> SMQEEDTFRELRIF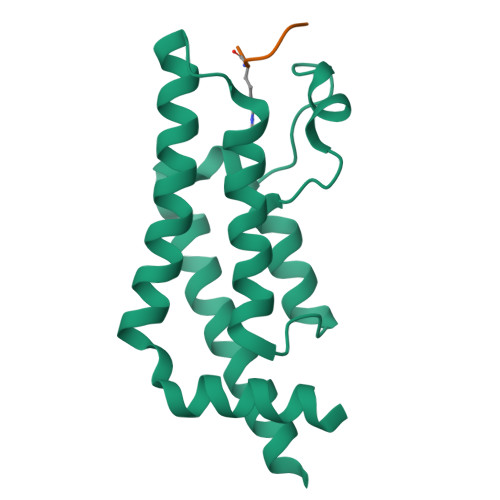LRNVTHRLAIDKRFRVFTKPVDPDEVPDYVTVIKQPMDLSSVISKIDLHKYLTVKDYLRDIDLICSNALEYNPDRDPGDRLIRHRACALRDTAYAIIKEELDEDFEQLCEEIQESR;> SGRGKG>MKFTVEREHLLKPLQQVSGPLGGRPTLPILGNLLLQVADGTLSLTGTDLEMEMVARVALVQPHEPGATTVPARKFFDICRGLPEGAEIAVQLEGERMLVRSGRSRFSLSTLPAADFPNLDDWQSEVEFTLPQATMKRLIEATQFSMAHQDVRYYLNGMLFETEGEELRTVATDGHRLAVCSMPIGQSLPSHSVIVPRKGVI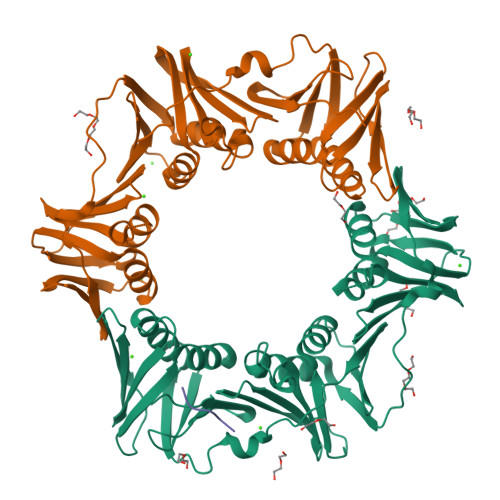ELMRMLDGGDNPLRVQIGSNNIRAHVGDFIFTSKLVDGRFPDYRRVLPKNPDKHLEAGCDLLKQAFARAAILSNEKFRGVRLYVSENQLKITANNPEQEEAEEILDVTYSGAEMEIGFNVSYVLDVLNALKCENVRMMLTDSVSSVQIEDAASQSAAYVVMPMRL[2x];> XQLDAF>GSMAGGVDGPIGIPFPDHSSDILSGLNEQRTQGLLCDVVILVEGREFPTHRSVLAACSQYFKKLFTSG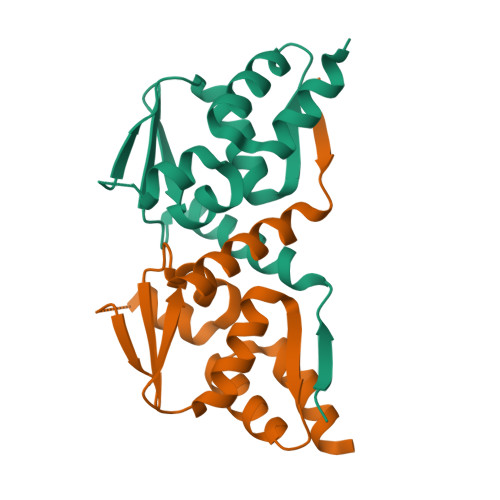AVVDQQNVYEIDFVSAEALTALMDFAYTATLTVSTANVGDILSAARLLEIPAVSHVCADLLDRQI[2x]>[3x]MPSVYGARLTTFEDEEKESEYGYVRKVSGPVVIADGMNGAAMYELVRVGHDNLIGEIIRLEGDSATIQVYEETAGLMVNDPVLRTHKPLSVELGPGILGNIFDGIQRPLKTIAIRSGDVYIPRGVSVPALDKDTLWEFQPKKIGEGDLLTGGDLYATVFENSLMQHHVALPPDAMGKVTYVAPAGQYSLKDTVLELEFQGVKKSFTMLQAWPVRTPRPVSSKLAADTPLLTGQRVLDALFPSVLGGTCAIPGAFGCGKTVISQALSKYSNSDTVVYVGCGERGNEMAEVLMDFPQLTMTLPDGREESVMKRTTLVANTSNMPVAAREASIYTGITIAEYFRDMGYNVSMMADSTSRWAEALREISGRLAEMPADSGYPAYLAARLASFYERAGKVKCLGGPERTGSVTIVGAVSPPGGDFSDPVTSATLSIVQVFWGLDK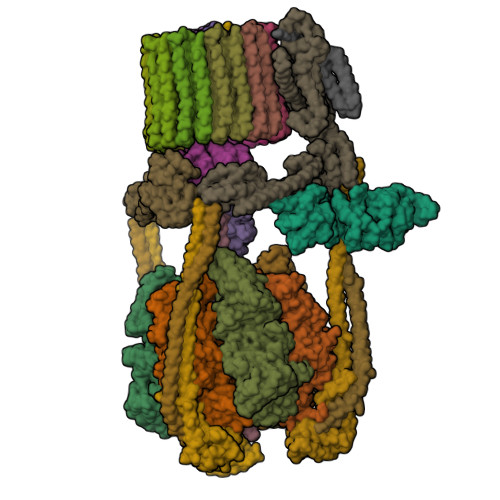KLAQRKHFPSVNWLISYSKYSTALESFYEQFDPDFINIRTKAREVLQREDDLNEIVQLVGKDALAEGDKITLETAKLLREDYLAQNAFTPYDKFCPFYKSVWMMRNIIHFYNLANQAVEKGAGMDGQKITYTLIKHRLGDLFYRLVSQKFEDPAEGEPALVAKFKKLHEDLTAGFRALEDETR;>MGVAQNNVDMEEGTLEVAMEYRTVTGVAGPLVILDKVKGPKYYEIVNIRLGDGTMRRGQVLEVDGEKAVVQVFEGTSGIDNKFTTVQFTGEVLKTPVSLDMLGRIFNGSGKPIDNGPPILPEAYLDISGSSINPSERTYPEEMIQTGISTIDVMNSIARGQKIPLFSAAGLPHNEIAAQICRQAGLVKRLEKTDNLLEDGEEDNFAIVFAAMGVNMETAQFFKRDFEENGSMERVTLFLNLANDPTIERIITPRIALTTAEYLAYECGKHVLVILTDMSSYADALREVSAAREEVPGRRGYPGYMYTDLAQIYERAGRIEGRKGSITQIPILTMPNDDITHPTPDLTGYITEGQIYIDRQLQNRQIYPPINVLPSLSRLMKSAIGEGMTRRDHSDVSNQLYANYAIGKDVQAMKAVVGEEALSSEDLLYLEFLDKFERKFVAQGAYDSRNIFQSLDLAWTLLRIFPRELLHRIPGKTLDQYYSRDAAN[3x];>[3x]MNDADVSKQIQQMVRFIRQEAEEKANEISVSAEEEFNIEKLQLVEAEKKKIRQEYERKEKQVEIRKKIEYSMQLNASRIKVLQAQDDLVSNMMEAASKEVLNVSRDHNSYKKLLKGLIVQSLLRLKEPAVLLRCRKDDHHLVESVLESAKEEYAQKLQVHPPEIIVDHHIYLPPGPGHHNAHGPSCSGGVVVASRDGKIVCENTLDARLDVVFRKKLPEIRKQLVSQVAA;>MASNRGHGGIQQLLAAEQEAQHIVAAARNAKMARLRQAKEEAEREIAEHRAQVEREFQRKLAESSGDSGANVKRLEQETEVKIHHLNAGAEKIQYDVVQMLLKHVTTVKN[3x];> MAQNQRLTVVPTVTMLGVMKSRLVGATRGHALLKKKSDALTVQFRQILKNIVTTKESMGEVMKDSSFALIEAKYVAGENIKHIVLENVQNASIKVRSRQENIAGVKIPKFEYFTDGETKNDLTGLARGGQQVQQCRAAYVKAIELLVELASLQTSFLTLDEAIKTTNRRVNALENVVKPRLENTITYIKGELDELEREDFFRLKKIQGYKKREIERQLASSKQFVEEQFAEKVSLQKGISIKSAQNLLSAGEKDEDIIF;> MAGRAQIPTKSSALIAMIADEDTVTGFLLAGVGNVDLRRKTNYLIVDSKTTVKAIEDAFKEFTTKEDIAIVLISQYVANMIRFLVDSYNKPIPAILEIPSKDHPYDPAHDSVLSRVKNLFSAESVASGRR;> MASRYWVVSLPVQNSAASVWNRLQEQISKHSFDTPLYRFNIPNLRVGTLDSLLALSDDLVKSNSFVESVSHKIRRQIEELERVSGIESSSLSVDGVPVDTYLTRFVWDEAKYPTMSPLREIVDGIHTLVAKIEDDLKVRVAEYNNVRSQLNAINRKQSGSLAVRDLSNLVKPEDIITSEHLVTLLAVVPKYSQKDWLASYETLTSYVVPRSSKLLYEDNEYALYTVTLFGRVADNFRIAAREKGFQIRDFEYSSEAQESRNQELEKLVHDQESLRSSLLQWCYTSYGEVFSSWMHFCAVRVFAESILRYGLPPSFLACVLAPSVKGEKKVRSILEELCGNANSTFWKSEDDGGMMAGLGGDADSHPYVSFTINLV;> MDHAELTTEQVLKRDIPWETYMTTKLISGTGLQLLRRYDNRSESHRAQLLDDDGPSYVRVFVSILRDIYKEETVEYVLALIDEMLTANPKRARLFHDKSLASEDTYEPFLRLLWKGNWFIQEKSCKILASIVSARPKPQDRFFANGEASNSKSKSTTIDDVLKLLVEWLCAQLKKPSHPSRGVPVAINCLAALLKEPMVRSSFVQADGVKLLTPLISPASTQQSIQLLYETCLCVWLLSYYEPAVEYLATTRTLPRLIDVVKSSTKEKVVRVVVLILRNLLPKGNFAAQMIDLGLPQVVQSLKAQAWSDEDLLEGLNQLEEGLKDNIKRLSSFDKYKQEVLLGHLDWSPMHKDPLFWRDNITNFEENDFQILRVLLTILDTSSDPRALAVACFDLSQFIQYHPAGRVIVTDLKAKERVMKLMNHENTEVTKSALLCIQRLFLGAKYASFLQA;> MAELQSGGGGGCCPPMDLFRSEPMQLVQIIIPIESAHLTVSYLGELGLLQFKDLNSEKSPFQRTYAAQIKKCAEMARKLRFFKEQMLKAGILSSVKSTTRADNNTDDLEVKLGDLEAELVEINANGDKLQRAHSELVEYKLVLQKAGEFFSSALTSAAAQQREMESQQTGEMTIETPLLTDKEMSADPSKQIKLGFIAGLVPREKSMSFERMLFRATRGNVFLRQAVVDEPVVDPVSGEKMEKNVFVVFYSGERAKNKILKICDAFGANRYPFNEEFDKQAQAISEVSGRLSELKTTLDAGLLHRGNLLQTIGDQFEQWNLLVKREKSIYHTLNMLSLDVTKKCLVGEGWSPVFATKQIQDALERAAFDSNSQVGAIFQVLHTKESPPTYFRTNKFTSAFQEIVDAYGVAKYREANPGVFTIVTFPFLFAVMFGDWGHGICLLLGTLVLIVREKKLASQKLDDITDMTFGGRYVILMMALFSIYTGLIYNEFFSVPFEIFSHSAYACRDLSCSEATTVGLIKVRDTYPFGVDPVWHGSRSELPFLNSLKMKMSILLGVAQMNLGIILSYFNATFFRIGVNIWCQFIPQIIFLNSLFGYLSLLIILKWITGSQADLYHVMIYMFLSPTDELGDNQLFPGQKTAQLVLLLLAFVSVPWMLLPKPFILKMQHQDRHQGQSYEALQSTDESLQPDTNHDSHGHEEFEFSEVFVHQMIHTIEFVLGAVSNTASYLRLWALSLAHSELSSVFYEKVLLLAWGYNNILILIVGIIVFIFATVGVLLVMETLSAFLHALRLHWVEFQNKFYEGDGYKFSPFSFALLDDEDE;> MSGSVMLGESSSWSRALVKISPYTFSAIGIAVAIGVSVLGAAWGIYITGSSLIGAAIKAPRITSKNLISVIFCEAVAIYGVIVAIILQTKLESVPASQIYAPESLRAGYAIFASGIIVGFANLVCGLCVGIIGSSCALSDAQNSSLFVKILVIEIFGSALGLFGVIVGIIMSAQASWPAKPV;> MYGFEAMTFNIHGGYLEAIVRGYRAGLLTAADYNNLCQCETLDDIKMHLSATEYGPYLQNEPSPLHTTTIVEKCTLKLVDEYKHMLCQATEPLSTFLEYITYGHMIDNVVLIVTGTLHERDVQELLEKCHPLGMFDSIATLAVAQNMRELYRLVLVDTPLAPYFSECITSEDLDDMNIEIMRNTLYKAYLEDFYKFCQKLGGATAEIMSDLLAFEADRRAVNITINSIGTELTRDDRRKLYSNFGLLYPYGHEELAVCEDIDQVRGVMEKYPPYQSIFSKLSYGESQMLDKAFYEEEVKRLCLAFEQQFHYGVFFAYMRLREQEIRNLMWISECVAQNQKSRVHDSVVFIF;> MGFLVTTLVFLVIGIIASLCTRICCNRGPSTNLLHLTLVITATVSCWMMWAIVYLAQMKPLIVPILSEEE;>[9x]MSTFSGDETAPFFGFLGAAAALVFSCMGAAYGTAKSGVGVASMGVMRPELVMKSIVPVVMAGVLGIYGLIIAVIISTGINPKAKSYYLFDGYAHLSSGLACGLAGLSAGMAIGIVGDAGVRANAQQPKLFVGMILILIFAEALALYGLIVGIILSSRAGQSRAE> HHHHHHMVTQFKTASEFDSAIAQDKLVVVDFYATWCGPCKMIAPMIEKFSEQYPQADFYKLD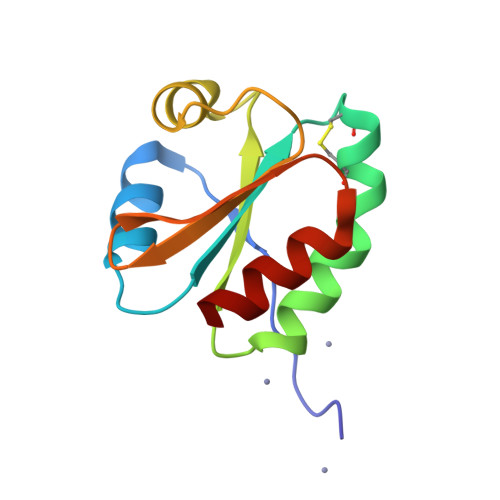VDELGDVAQKNEVSAMPTLLLFKNGKEVAKVVGANPAAIKQAIAANA~{N},~{N}-dimethyl-2-[4-[4-(2,6-naphthyridin-4-yl)phenyl]pyrazol-1-yl]ethanamide | C21 H19 N5 O | 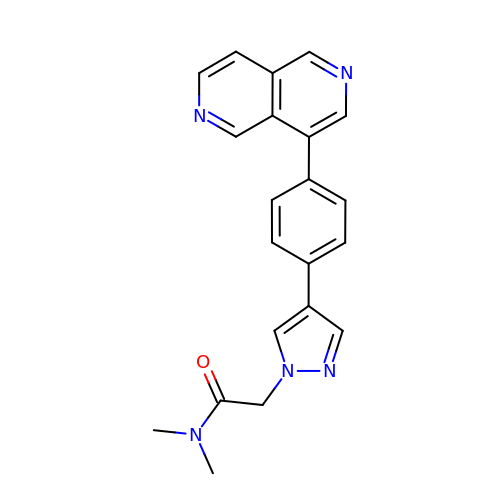OQOHDKVDMBADIN-UHFFFAOYSA-N>DSVTQTEGQVALSEEDFLTIHCNYSASGYPALFWYVQYPGEGPQFLFRASRDKEKGSSRGFEATYNKEATSFHLQKASVQESDSAVY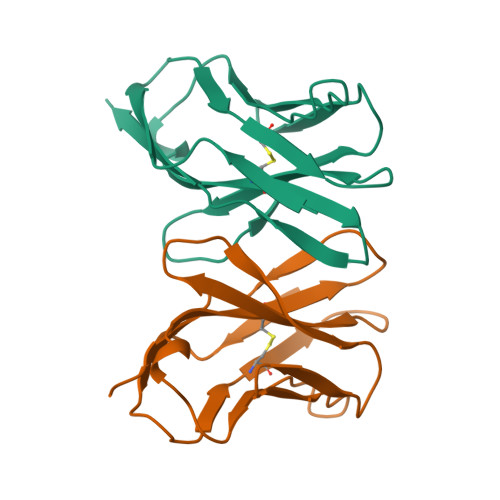YCALSGGNNKLTFGAGTKLTIKP[2x]> GAMGVNVLASTVSGAIERLGLTYEEVGDIVDASPRSVARWTAGQVVPQRLNKQRLIELAYVADALAEVLPRDQANVWMFSPNRLLEHRKPADLVRDGEYQRVLALIDAMAEGV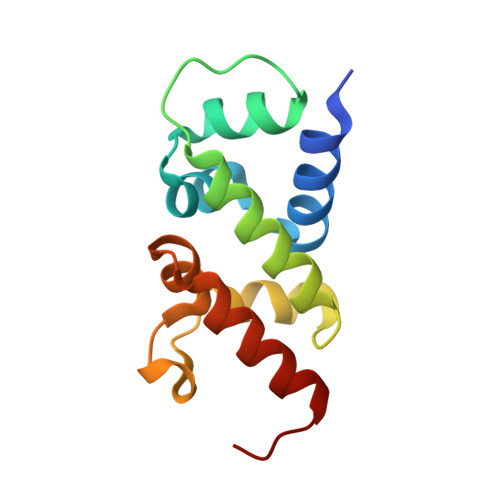FV> DWNNQSIVKTGERQHGIHIQGSDPGGVRTASGTTIKVSGRQAQGILLENPAAELQFRNGSVTSSGQLSDDGIRRFLGTVTVKAGKLVADHATLANVGDTWDDDGIALYVAGEQAQASIADSTLQGAGGVQIERGANVTVQRSAIVDGGLHIGALQSLQPEDLPPSRVVLRDTNVTAVPASGAPAAVSVLGASELTLDGGHITGGRAAGVAAMQGAVVHLQRATIRRGDALAGGAVPGGAVPGGAVPGGFGPGGFGPVLDGWYGVDVSGSSVELAQSIVEAPELGAAIRVGRGARVTVPGGSLSAPHGNVIETGGARRFAPQAAPLSITLQAGAHAQGKALLYRVLPEPVKLTLTGGADAQGDIVATELPSIPGTSIGPLDVALASQARWTGATRAVDSLSIDNATWVMTDNSNVGALRLASDGSVDFQQPAEAGRFKVLTVNTLAGSGLFRMNVFADLGLSDKLVVMQDASGQHRLWVRNSGSEPASANTLLLVQTPLGSAATFTLANKDGKVDIGTYRYRLAANGNGQWSLV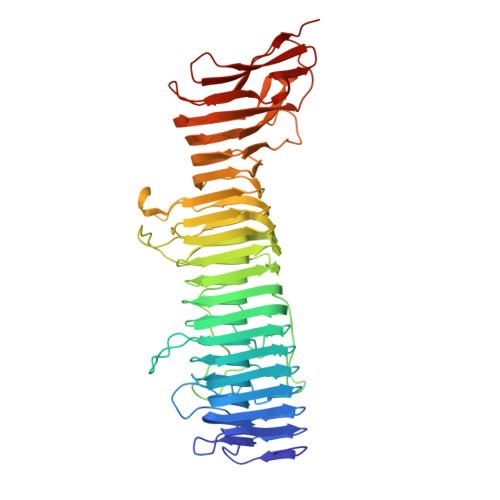GAKAPP> MKTVVIGAGLGGLLSAARLSKAGHEVEVFERLPITGGRFTNLSYKGFQLSSGAFHMLPNGPGGPLACFLKEVEASVNIVRSEMTTVRVPLKKGNPDYVKGFKDISFNDFPSLLSYKDRMKIALLIVSTRKNRPSGSSLQAWIKSQVSDEWLIKFADSFCGWALSLKSDEVPVEEVFEIIENMYRFGGTGIPEGGCKGIIDALETVISANGGKIHTGQEVSKILIENGKA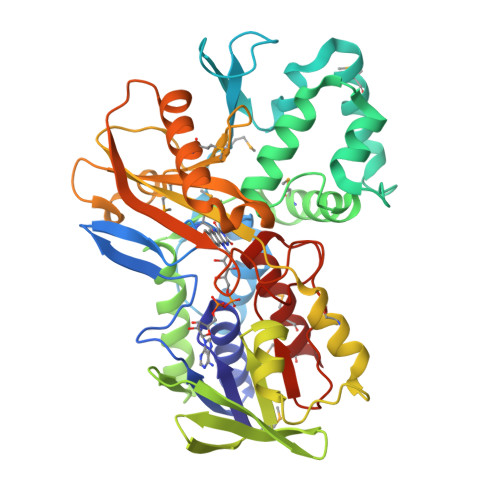AGIIADDRIHDADLVISNLGHAATAVLCSEALSKEADAAYFKMVGTLQPSAGIKICLAADEPLVGHTGVLLTPYTRRINGVNEVTQADPELAPPGKHLTMCHQYVAPENVKNLESEIEMGLEDLKEIFPGKRYEVLLIQSYHDEWPVNRAASGTDPGNETPFSGLYVVGDGAKGKGGIEVEGVALGVMSVMEKVLG>DLWQFGKMILKETGKLPFPYYVTYGCYCGVGGRGGPKDATDRCCFVHDCCYGKLTSCKPKTDRYSYSRKDGTIVCGENDPCRKEICECDKAAAVCF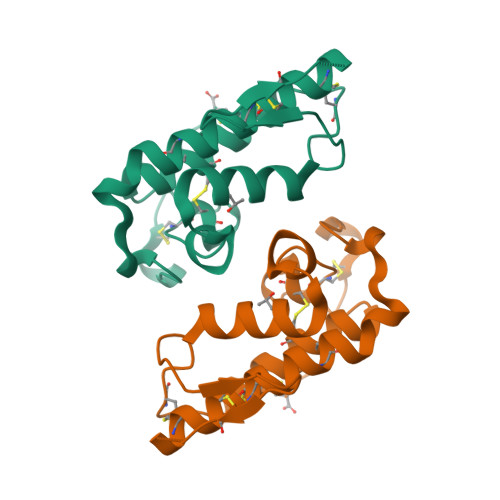RENLDTYNKKYMSYLKSLCKKXADDC[2x]Ito et al. showed that cereblon associates with damaged DNA binding protein 1 (DDB1) to act as a substrate receptor for the DDB1/cullin4 E3 ubiquitin ligase complex. In mammals, cereblon has a LON domain and a C-terminal thalidomide binding domain. However, homologs of the latter, also termed the CULT domain, are further found in animals and bacteria as single-domain proteins, that have all essential residues of the thalidomide binding site conserved. Architecturally, the thalidomide binding domain is a member of the β-tent fold, which consists of two antiparallel beta sheets that are oriented at an approximately right angle and pinned together at the top via a structural zinc ion.

As we have so far not been able to crystallize MsCI4 in the absence of ligands, we tried the following prolonged soaking experiment: We soaked crystals of the original orthorhombic crystal form of MsCI4•thalidomide for many hours in the cryo-protectant solution in order to “wash out” thalidomide from the binding sites. Diffraction experiments were performed with crystals from two different crystallization conditions after 40 h of washing. In the two resulting structures, thalidomide was retained in two of the three monomers in the ASU, but released in the third monomer. Strikingly, the loss of the ligand was accompanied by the unfolding of a large portion of the protein around the binding site. In one of the structures, “Wash II”, three regions totaling to 37% of the previously structured part of the main chain were no longer traceable in the electron density. The largest is the most N-terminal unfolded region, which starts between β2 and β3 and comprises the hairpin formed by β3 and β4, leaving only a C-terminal remainder of β4. The second region starts in the middle of β5, comprises the first tryptophan of the aromatic cage, and ends at the cage’s second tryptophan at the start of β6, rendering its indole side chain disordered. The third and smallest region is the loop connecting β7 and β8. Therein we find a minimal invariant consensus structure that exactly coincides with the structured part of the “Wash II” structure: While the three flexible regions derived from the washing experiment are found in a multitude of conformations, the remainder of the protein is essentially invariant in all structures.

>[3x]AMPLDAGGQNSTQMVLAPGASIFRCRQCGQTISRRDWLLPMGGDHEHVVFNPAGMIFRVWCFSLAQGLRLIGAPSGEFSWFKGYDWTIALCGQCGSHLGWHYEGGSQPQTFFGLIKDRLAEGPAD>SFASTSGLQFTIDGETGYFAGTNSYWIGFLTDNADVDLVMGHLKSSGLKILRVWGFNDVTSQPSSGTVWYQLHQDGKSTINTGADGLQRLDYVVSSAEQHDIKLIINFVNYWTDYGGMSAYVSAYGGSGETDFYTSDTMQSAYQTYIKTVVERYSNSSAVFAWELANEPRCPSCDTSVLYNWIEK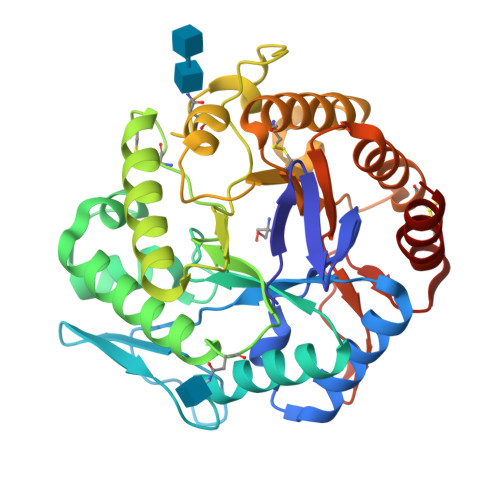TSKFIKGLDADRMVCIGDEGFGLNIDSDGSYPYQFSEGLNFTMNLDIDTIDFGTLHLYPDSWGTSDDWGNGWITAHGAACKAAGKPCLLEEYGVTSNHCSVEGAWQKTALSTTGVGADLFWQYGDDLSTGKSPDDGNTIYYGTSDYQCLVTDHVAAIGSA[2x]> AAGVAAWLPFARAAAIGWMPVASGPMPAPPRQERKRTQDALIVLNVSGTRFQTWQDTLERYPDTLLGSSERDFFYHPETQQYFFDRDPDIFRHILNFYRTGKLHYPRHECISAYDEELAFFGLIPEIIGDCCYEEYKDRRRENAERLQDDADTDTAGESALPTMTARQRVWRAFENPHTSTMALVFYYVTGFFIAVSVIANVVETVPCGSSPGHIKELPCGERYAVAFFCLDTACVMIFTVEYLLRLAAAPSRYRFVRSVMSIIDVVAILPYYIGLVMTDNEDVSGAFVTLRVFRVFRIFKFSRHSQGLRILGYTLKSCASELGFLLFSLTMAIIIFATVMFYAEKGSSASKFTSIPAAFWYTIVTMTTLGYGDMVPKTIAGK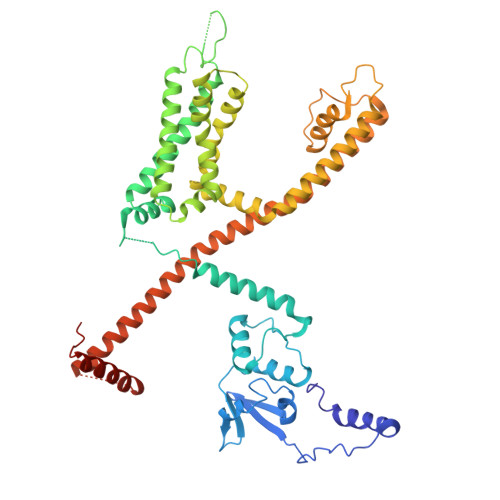IFGSICSLSGVLVIALPVPVIVSNFSRIYHQNQRADKRRAQKKARLARIRAAKSGSANAYMQSKRSGLLSNQGRGDGSAFVTKSGSSFETQHHHLLHCLEKTTNHEFVD>[2x]MERAEILGVGTELLYGETLDTNTAEIARSLKPYALKVERTLRVADEVAPLAREVEEAFARARLVVLSGGLGPTPDDVTREAVALALGEPLELDEAVLGEIEAFFRARGRAMPEANRKQAMRIPSATWLKNPRGTAPGWWVRKGGKDLVLLPGPPPEWRPMWQEVLPRLGLPRRPYAERVLKTWGIGESEIVERLGPLFVRGEEVEVGTYPKVHGVEVVVRGREDRVAELAERIKKKLLKEVWGEGEMTLAEAVKRRMEREGATLSTMESLTGGLLGAEITRVPGASRFYLGGVVSYSVGAKARFGVPQDLLSRTVSAETARAMAEAARSLFGSTYALATTGVAGPDPLEGEPPGTVYVALAGPTGAEVRRYRFPGDRETVRLRSVYAALALLVT

Here we describe the determination of the crystal structure of CinA from T. thermophilus (TtCinA), which contains both the NMN deamidase and COG1058 domains and is therefore a bifunctional enzyme. In addition, we show that TtCinA adopts a three-domain structure, with a third, previously unidentified, KH-type domain between the NMN deamidase and COG1058 domains. We demonstrate that TtCinA adopts an asymmetric dimer and present structures with NCN, ADP-ribose, AMP, and ATP bound, which provide experimental validation for the modes of substrate binding proposed previously. We use these structures to propose models for both enzymatic activities and suggest that large scale movement of the COG1058 domains is linked to ADPR catalysis as well as providing a rationale for the usual asymmetric arrangement of the TtCinA dimer.

Data were collected from three different complexes, following soaking of TtCinA crystals with ADP-ribose, ATP, and AMP/ribose 5-phosphate. Both the ADP-ribose and ATP data sets produced clear difference density in both catalytic sites (top and central panels). Examination of the recognition of ADP-ribose in the open binding site (chain A) showed a hydrogen bond from Asp-20 to the adenine ring. A strong peak in the electron density map, inferred to be from Mg2+, was identified between the α and β phosphates. Such a location would be consistent with pyrophosphatase activity. Asp-76 binds the Mg2+ ion and is absolutely conserved in CinA sequence alignments. Glu-156 appears to play an important part in recognition of the terminal ribose ring; it forms two hydrogen bonds to the 2′- and 3′-hydroxyl groups in the ribose ring and is also absolutely conserved in sequence alignments. Recognition of ADP-ribose in the closed site is very similar to that in the open but with the important exception that there are additional points of contact between the ligand and TtCinA from residues in the KH domain of chain A. The side chain of Lys-211 and the carbonyl oxygen of Pro-210 form hydrogen bonds to the 2′- and 3′-hydroxyl groups in the ribose moiety in the ADP part of the molecule. In addition, the binding of the Mg2+ ion appears to be stabilized by Glu-187, which extends from the end of an α-helix in the KH domain into the ADP-ribose binding site. Conversely, the closed site is more likely to correspond to the catalytically competent state; critically, the close approach of the KH domain from chain A, with Glu-187, would promote the binding of Mg2+ and hence polarize the P=O bond for hydrolysis. A major feature of the TtCinA structure is the asymmetry in the dimer, which is caused by contact between a KH-type domain on the opposite chain and the bound ADP-ribose.>[2x]GMKTTEYVAEILNELHNSAAYISNEEADQLADHILSSHQIFTAGAGRSGLMAKSFAMRLMHMGFNAHIVGEILTPPLAEGDLVIIGSGSGETKSLIHTAAKAKSLHGIVAALTINPESSIG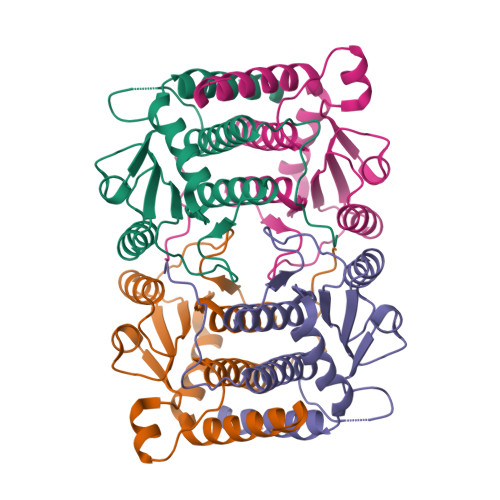KQADLIIRMPGSPKDQSNGSYKTIQPMGSLFEQTLLLFYDAVILKLMEKKGLDSETMFTHHANLE> GKQFRQIAKVPYRVLDAPSLADDFYYSLIDWSSTDVLAVALGKSIFLTDNNTGDVVHLCDTENEYTSLSWIGAGSHLAVGQANGLVEIYDVMKRKCIRTLSGHIDRVACLSWNNHVLTSGSRDHRILHRDVRMPDPFFETIESHTQEVCGLKWNVADNKLASGGNDNVVHVYEGTSKSPILTFDEHKAAVKAMAWSPHKRGVLA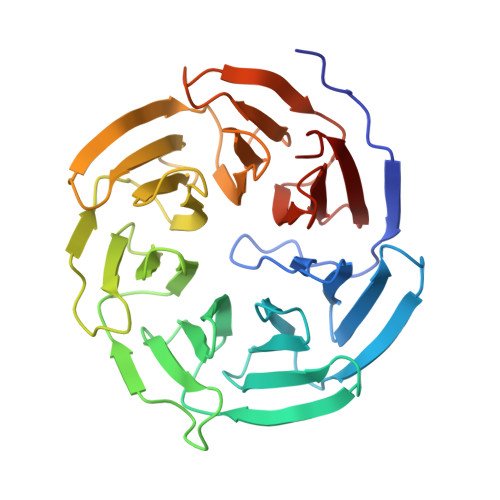TGGGTADRRLKIWNVNTSIKMSDIDSGSQICNMVWSKNTNELVTSHGYSKYNLTLWDCNSMDPIAILKGHSFRVLHLTLSNDGTTVVSGAGDETLRYWKLFDKP> HPETLVKVKDAEDQLGARVGYIELDLNSGKILESFRPEERFPMMSTFKVLLCGAVLSRIDAGQEQLGRRIHYSQNDLVEYSPVTEKHLTDGMTVRELCSAAITMSDNTAANLLLTTIGGPKELTAFLHNMGDHVTRLDRWEPELNEAIPNDERDTTMPVAMATTLRKLLTGELLTLASRQQLIDWM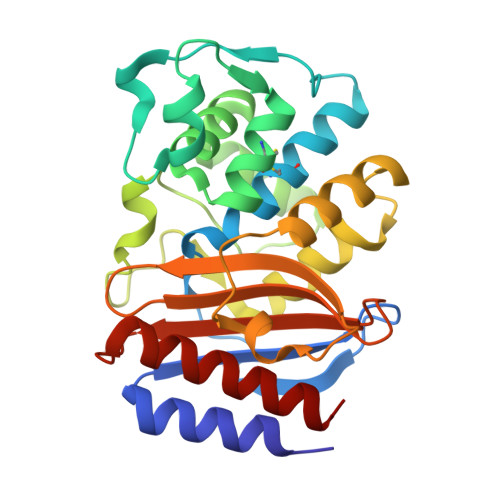EADKVAGPLLRSALPAGWFIADKSGAGERGSRGIIAALGPDGKPSRIVVIYTTGSQATMDERNRQIAEIGASLIKHW>[3x]AQVI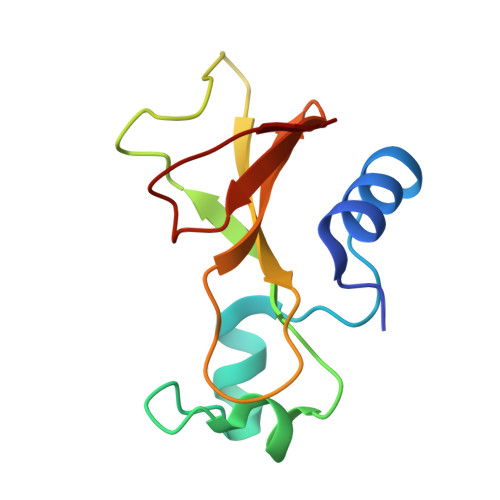NTFDGVADYLQTYHKLPDNYITKSEAQALGWVASKGNLADVAPGKSIGGDIFSNREGKLPGKSGRTWREADINYTSGFRNSDRVLYSSDWLIYKTTDHYQTFTKIR>SNAMEKYILSIDQGTTSSRAILFNQKGEIAGVAQREFKQYFPQSGWVEHDANEIWTSVLAVMTEVINENDVRADQIAGIGITNQRETTVVWDKHTGRPIYHAIVWQSRQTQSICSELKQQGYEQTFRDKTGLLLDPYFAGTKVKWILDNVEGAREKAENGDLLFGTIDTWLVWKLSGKAAHITDYSNASRTLMFNIHDLEWDDELLELLTVPKNMLPEVKASSEVYGKTIDYHFYGQEVPIAGVAGDQQAALFGQACFERGDVKNTYGTGGFMLMNTGDKAVKSESGLLTTIAYGIDGKVNYALEGSIFVSGSAIQWLRDGLRMINSAPQSESYATRVDSTEGVYVVPAFVGLGTPYWDSEARGAIFGLTRGTEKEHFIRATLESLCYQTRDVMEAMSKDSGIDVQSLRVDGGAVKNNFIMQFQADIVNTSVERPEIQETTALG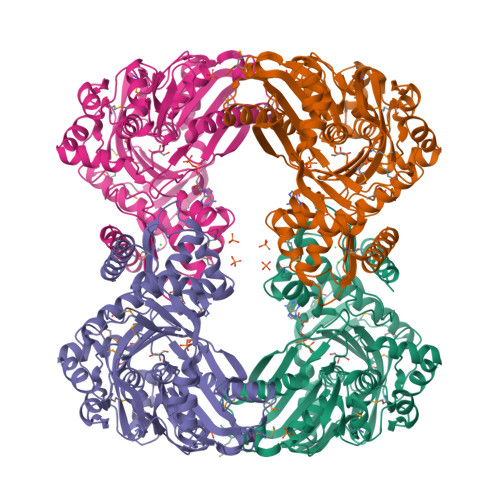AAFLAGLAVGFWESKDDIAKNWKLEEKFDPKMDEGEREKLYRGWKKAVEATQVFKTE[4x]ExbB and ExbD are cytoplasmic membrane proteins that associate with TonB to convey the energy of the proton-motive force to outer membrane receptors in Gram-negative bacteria for iron uptake. The opportunistic pathogen Serratia marcescens (Sm) possesses both TonB and a heme-specific TonB paralog, HasB. ExbBSm has a long periplasmic extension absent in other bacteria such as E. coli (Ec). We purified ExbBSm alone and ExbBDSm and determined their structures by single-particle cryo-EM at 3.1 and 3.96 Å resolution, respectively.

Due to this strong bias in particle orientation, the resolution achieved was 3.96 Å, precluding reliable positioning of the side chains. As observed for ExbBSm alone, in the ExbBDSm complex, ExbBSm behaves as a pentamer, and no sign of other assemblies was found. Similarly, no density could be attributed to the periplasmic extension. Two clear densities inside the ExbBSm pore were assigned to the pair of ExbDSm TM segments. In the refined model, Asp 25 from ExbDSm monomer chain G faces Thr 218 from ExbBSm chain C, while Asp 25 from the ExbDSm chain F faces the interface between two ExbBSm monomers A and E. As compared to the structure of ExbBSm, there is a slight «opening» towards the periplasmic side (the distance of Ala 197 from one subunit to Leu 204 of the facing subunit varying from 25.5 Å in ExbBSm to 29.8 Å in ExbBDSm, much greater than any error expected due to the difference in resolution of the two structures). This opening of the structure is limited to the periplasmic part. In summary, we show that ExbBD from S. marcescens has a 5:2 stoichiometry with a larger channel allowing solvent or proton transport from the periplasmic side as compared with the E. coli structure.

>APAANPAVTESVAPTTAPAPAAAAPESITPVNPAPTIQPPETRGMDLSIWGMYQHADAVVKAVMIGLVLASIVTWTILFAKGSELLRAKRRLRREQLALAEARSLDEASELAQNFSPESVSAVLLNDAQNELELSAESNDNNGIKERTGFRLERRVAAYSRNMGRGNGFLATIGAISPFVGLFGTVWGIMNSFIGIAHSQTTNLAVVAPGIAEALLATAMGLVAAIPAVVIYNIFARVISGHRAQVGDVAAQVLLLQGRDLDLAATAEAKRSQHAHQLRAG[5x];>[2x]MAMRLNEDLDDSGELHEINVTPFIDVMLVLLIIFMVAAPLATVDIRVDLPASSAKPQPRPEKPVFLSVKADKQLYVGDQPVNADQLTSVLDQRTQANKETTIFFQADKSVDYETLMSVMDTLRKAGYLKVGLVGMEGAAKHHHHHH> MGLEEKKENKQLTYTTVKDIGDMNPHVYGGSMSAESMIYEPLVRNTKDGIKPLLAKKWDVSEDGKTYTFHLRDDVKFHDGTPFDADAVKKNIDAVQENKKL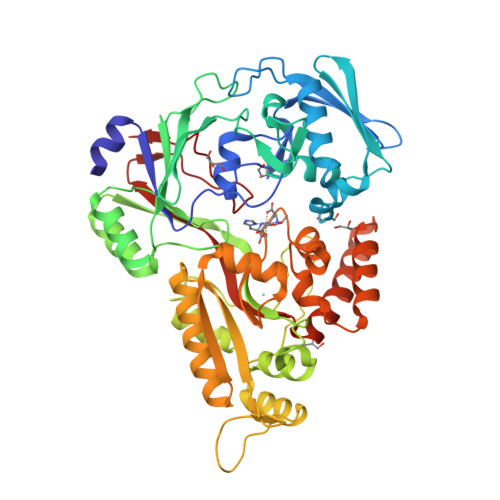HSWLKISTLIDNVKVKDKYTVELNLKEAYQPALAELAMPRPYVFVSPKDFKNGTTKDGVKKFDGTGPFKLGEHKKDESADFNKNDQYWGEKSKLNKVQAKVMPAGETAFLSMKKGETNFAFTDDRGTDSLDKDSLKQLKDTGDYQVKRSQPMNTKMLVVNSGKKDNAVSDKTVRQAIGHMVNRDKIAKEILDGQEKPATQLFAKNVTDINFDMPTRKYDLKKAESLLDEAGWKKGKDSDVRQKDGKNLEMAMYYDKGSSSQKEQAEYLQAEFKKMGIKLNINGETSDKIAERRTSGDYDLMFNQTWGLLYDPQSTIAAFKAKNGYESATSGIENKDKIYNSIDDAFKIQNGKERSDAYKNILKQIDDEGIFIPISHGSMTVVAPKDLEKVSFTQSQYELPFNEMQYK> LAFQ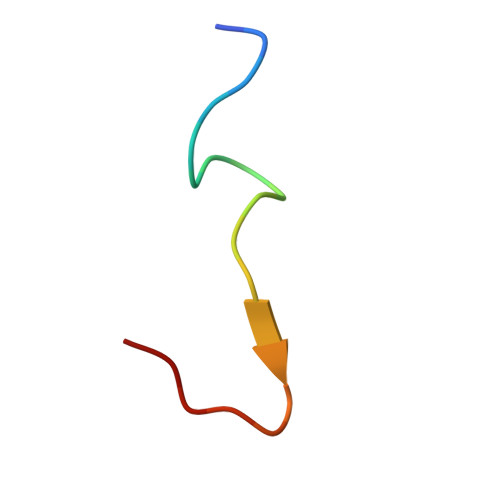REGFGRQSMSEKRTKQ> MQNGYTYEDYQDTAKWLLSHTEQRPQVAVICGSGLGGLVNKLTQAQTFDYSEIPNFPESTVPGHAGRLVFGILNGRACVMMQGRFHMYEGYPFWKVTFPVRVFRLLGVETLVVTNAAGGLNP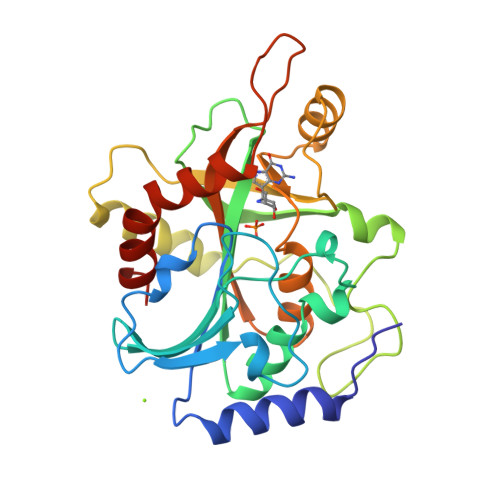NFEVGDIMLIRDHINLPGFSGENPLRGPNEERFGVRFPAMSDAYDRDMRQKAHSTWKQMGEQRELQEGTYVMLGGPNFETVAECRLLRNLGADAVGMSTVPEVIVARHCGLRVFGFSLITNKVIMDYESQGKANHEEVLEAGKQAAQKLEQFVSLLMASIPV>[2x]HHHHHHFNLPPGNYKKPKLLYCTTGHFLRILPD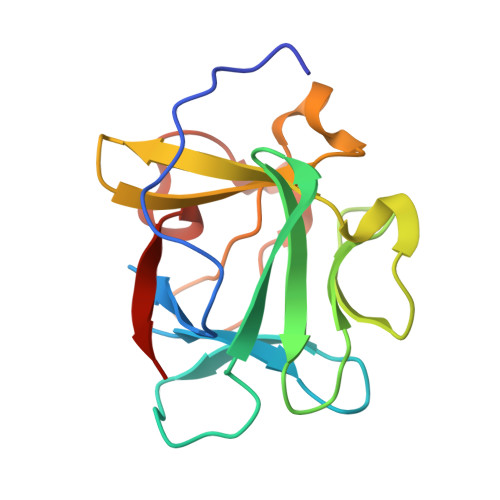GTVDGTRDRSDQHIQLQLSAESVGEVYIKSTETGQYLAMDTDGLLYGSQTPNEECLFLERLEENHYNTYISKKHAEKNWFVGLKKNGSCKRGPRTHYGQKAILFLPLPVSSD N-9-(1',2',3',4'-TETRAHYDROACRIDINYL)-1,8-DIAMINOOCTANE | C21 H33 N3 | 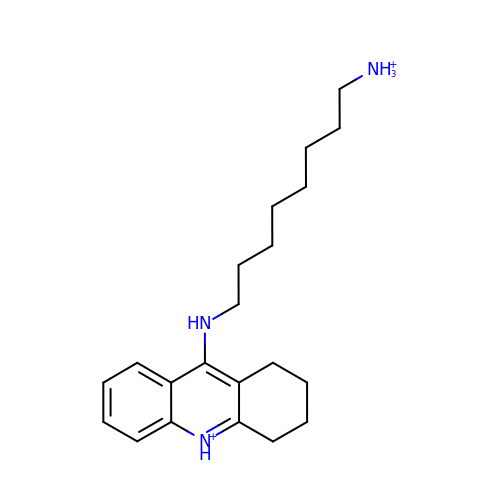LFBAUYQQFKFFCF-UHFFFAOYSA-P>AMKKDSKAPCVEVFDERDGCKAAGTQKASGDDGFCVKVSMKAIGFNAAEAASVTKNYGIKRFGAKSV[2x];>[2x]MLDAFSKVITSADGKAAYVGGADLQALKKFVSEGNKRMDSVNAIVSNASCIVSDSVSGMVCENPSLIAPNGGVYTNRKMAACLRDAEIILRYVSYSLLSGDSSVLEDRCLNGLKETYASLGVPAAGNARTISIMKATVIGFITNNSQQKKLSTPAGDCSALASEVGGYFDKVSSALA;>AMKKDSKAPCVEVFDERDGCKAAGTQKASGDDGFCVKVSMKAIKMNAAEATSVTKNYNTKLL[2x]

Cryptophyte algae have a unique phycobiliprotein light-harvesting antenna that fills a spectral gap in chlorophyll absorption from photosystems. We show that the cryptophyte Hemiselmis andersenii expresses an energetically complex antenna comprising three distinct spectrotypes of phycobiliprotein, each composed of two αβ protomers but with different quaternary structures arising from a diverse α subunit family. We report crystal structures of the major phycobiliprotein from each spectrotype. We propose that the macromolecular organization of the cryptophyte antenna consists of bulk open and open-braced forms that transfer excitations to photosystems via this bridging closed form phycobiliprotein.

Four new structures of HaPE555 were determined (resolutions: 1.57 Å, 1.67 Å, 1.73 Å and 1.95 Å). The largest peak of HaPE555 (555 A) is by far the most abundant PBP constituting approximately 63% of the overall protein complement (with other HaPE555 spectrotype peaks contributing 8%). All five crystal forms of protein HaPE555 are constructed from continuous filaments of PBPs, which are organized into two-dimensional rafts. The filaments are generated via knobs-into-holes packing but differ in the distances between adjacent molecules along the filament (having either tight or loose interfaces). This packing brings the chromophores of neighboring PBPs closer together increasing the possibility of energy transfer. The bulk antenna proteins, HaPE555 and HaPE560, are densely packed to form a concentrated glass of proteins as evidenced by electron micrographs and FRAP experiments. It is also possible that the rafts of HaPE555 filaments seen in all crystal forms are part of the organizing principle of the antenna architecture. We have shown that HaPE555 and HaPE560 form the bulk of the light harvesting antenna (roughly 6/7 of the PBPs) and capture the highest energy photons. Thus, HaPE555 and HaPE560 have evolved to capture photons that would be otherwise lost by the integral membrane photosystems: they plug a spectral hole.> KSLRVSSLNKDRRLLLREFYNLEN;> MN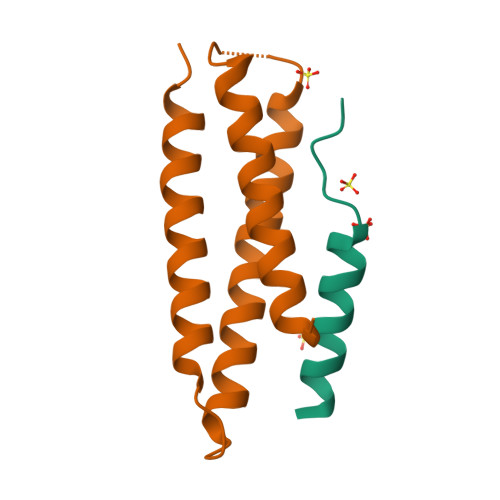NSEDPFQQVVKDTKEQLNRINNYITRHNTAGDDDQEEEIQDILKDVEETIVDLDRSIIVMKRDENEDVSGREAQVKNIKQQLDALKLRFDRRI The naphthyridine carbamate dimer (NCD) is a small molecule that recognizes disease-related RNA containing UGGAA repeats associated with spinocerebellar ataxia type 31 (SCA 31) and alleviates the disease phenotype in vitro and in vivo. SCA 31 is an autosomal spinocerebellar neurodegenerative disorder. It is caused by abnormally repeated 5′-UGGAA-3′/5′-UGGAA-3′ RNA pentads, which sequester many cellular proteins by forming toxic nuclear foci. Each of the oligomers formed self-complementary duplex: ROG1 (GGCACUGGAAGUGC)2 and ROG2 (GGCACUGGAAGUGCC)2; containing the 5′-UGGAA-3′/5′-UGGAA-3′ pentad motif selectively recognized by NCD. We crystallized two RNA–ligand complexes: ROG1–NCD (1.50 Å resolution) and ROG2–NCD (2.55 Å resolution) and one unliganded duplex of ROG2 oligomer (2.79 Å).

In the ROG1–NCD complex, a third ligand molecule was observed between the 5′ ends of the symmetry-related helices, participating in crystal lattice formation (vide section: Role of NCD ligand in crystal lattice formation). In the ROG1–NCD model, the third ligand molecule connected the symmetry-related RNA helices. The contacts in the crystal lattice were formed by two NCD molecules (one from the asymmetric unit and second, NCD’, from the symmetry-related complex) and four RNA duplexes (one from the asymmetric unit and three from symmetry-related RNAs). The NCD was bound to the 1G residue of chain B and 1G of chain A’. The observed lattice interactions resulted in the alignment of two helices, one above the other, while the other two helices were perpendicular to the RNA helix from the asymmetric unit. In the ROG1–NCD model, the aliphatic linker of the ligand connecting symmetry-related molecules showed a similar zigzag conformation but consisted of seven atoms (C14, C15, C16, N17, C16’, C15’, and C14’). This resulted in a longer distance (7.4 Å) between the two NU planes. Additionally, the NUs were twisted relative to each other by 17° and their nitrogen edges showed a trans geometry. The use of NCD as a “molecular glue” for crystal lattice formation may be more advantageous because it connects four RNA molecules instead of two, as in the case of overhanging nucleotides. This resulted in formation of crystal lattice in all directions and improved the data resolution from 2.55 Å (ROG2–NCD) to 1.5 Å for ROG1–NCD.

>GGCACUGGAAGUGC[2x]> YNLDVRGARSFSPPRAGRHFGYRVLQVGNGVIVGAPGEGNSTGSLYQCQSGTGHCLPVTLRGSNYTSKYLGMTLATDPTDGSILACDPGLSRTCDQNTYLSGLCYLFRQNLQGPMLQGRPGFQECIKGNVDLVFLFDGSMSLQPDEFQKILDFMKDVMKKLSNTSYQFAAVQFSTSYKTEFDFSDYVKWKDPDALLKHVKHMLLLTNTFGAINYVATEVFREELGARPDATKVLIIITDGEATDSGNIDAAKDIIRYIIGIGKHFQTKESQETLHKFASKPASEFVKILDTFEKLKDLFTELQKKIYVIEGTSKQDLTSFNMELSSSGISADLSRGHAVVGAVGAKDWAGGFLDLKADLQDDTFIGNEPLTPEVRAGYLGYTVTWLPSRQKTSLLASGAPRYQHMGRVLLFQEPQGGGHWSQVQTIHGTQIGSYFGGELCGVDVDQDGETELLLIGAPLFYGEQRGGRVFIYQRRQLGFEEVSELQGDPGYPLGRFGEAITALTDINGDGLVDVAVGAPLEEQGAVYIFNGRHGGLSPQPSQRIEGTQVLSGIQWFGRSIHGVKDLEGDGLADVAVGAESQMIVLSSRPVVDMVTLMSFSPAEIPVHEVECSYSTSNKMKEGVNITICFQIKSLIPQFQGRLVARLTYTLQLDGHRTRRRGLFPGGRHELRRNIA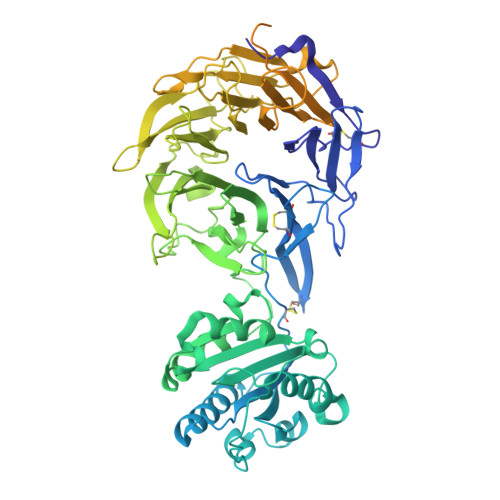VTTSMSCTDFSFHFPVCVQDLISPIRVSLNFSLWEEEGTPRDQRAQGKDIPPILRPSLHSETWEIPFEKNPAALQTLFQGPLGAQGEKELQALEKENAQLEWELQALEKELAQHHHHHHA> STQKSLSKEEIERYSRQMIVPGMGKEGQLRLMNAKVLIIGAGGLGCPAAQYLAGAGVGTIGIVDGDSVETSNLHRQVAHATKRVGMLKVDSLITHLIEINPLPVYVPYRFDLTPQNAAQIIKPWDVILDCTDNPATRYLISDVCVLLGKPLVSAASVQKSGQLIVLNCPPTPQG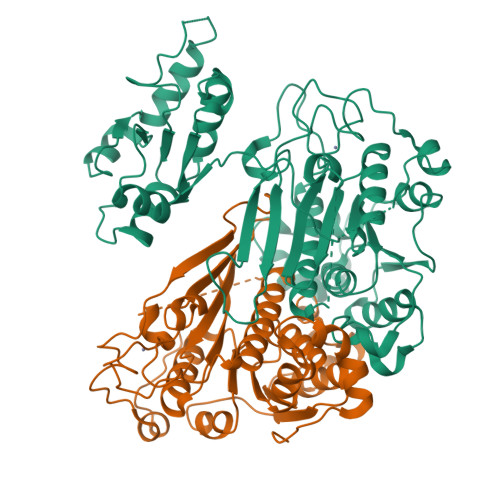VVNKKAAPCYRCCFKKPPPPSAQTSCGEAGIMGPVVGMMGVAQAGEAIKILVSQLHMPPKEGEEVSPEKNLVQPTLLIYTYDLNSAIGPYSFRALKMGGRKKDCFACGENSTLTLDGIKSGNPNYVQFCGNMTQSTNLAPEDRITATAYNEKRRNGELGEHILLDTREKEHFSFGSIPGAVNVPFSKFLVKASSIKREGNSPAELLPMQPASDEAPIVVVCRRGQDSQEVVEKLKELGLDNGGKRKIMDIVGGMKAWRDEVDPDFPFI;> GSTQKSLSKEEIERYSRQMIVPGMGKEGQLRLMNAKVLIIGAGGLGCPAAQYLAGAGVGTIGIVDGDSVETSNLHRQVAHATKRVGMLKVDSLITHLIEINPLPVYVPYRFDLTPQNAAQIIKPWDVILDCTDNPATRYLISDVCVLLGKPLVSAASVQKSGQLIVLNCPPTPQGVVNKKAAPCYRCCFKKPPPPSAQTSCGEAGIMGPVVGMMGVAQAGEAIKILVSQLHMPPKEGEEVSPEKNLVQPTLLIYTYDLNSAIGPYSFRALKMGGRKKDCFACGENSTLTLDGIKSGNPNYVQF;> DRITATAYNEKRRNGELGEHILLDTREKEHFSFGSIPGAVNVPFSKFLVKASSIKREGNSPAELLPMQPASDEAPIVVVCRRGQDSQEVVEKLKELGLDNGGKRKIMDIVGGMKAWRDEVDPDFPFI> MGSSQITFNTTQQGDMYTIIPEVTLTQSCLCRVQILSLREGSSGQSQTKQEKTLSLPANQ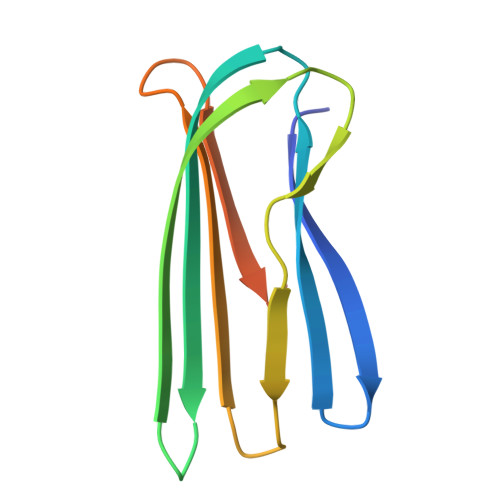PIALTKLSLNISPDDRVKIVVTVSDGQSLHLSQQWPPSSEKSLEHHHHHH>[2x]HMASREQTMENILKAAKKKFGERGYEGTSIQEIAKEAKVNVAMASYYFNGKENLYYEVFKKYGLANELPNFLEKNQFNPINALREYLTVFTTHIKENPEIGTLAYEEIIKESARL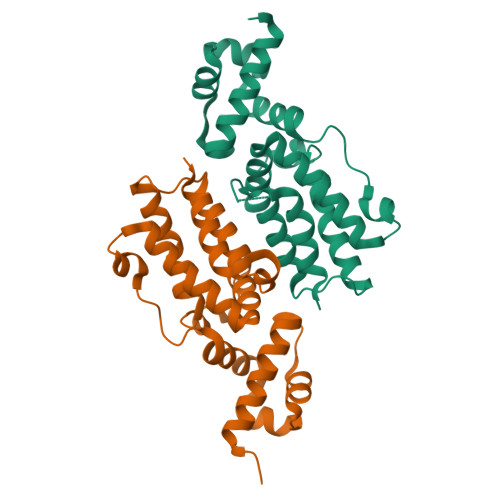EKIKPYFIGSFEQLKEILQEGEKQGVFHFFSINHTIHWITSIVLFPKFKKFIDSADLVSRIISALTDKPNI(3~{R})-8-methoxy-3-methyl-3-oxidanyl-2,4-dihydrobenzo[a]anthracene-1,7,12-trione 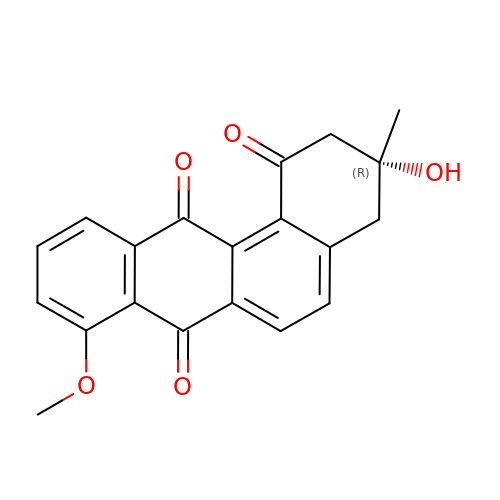| C20 H16 O5 | XZLGWJORNHETKI-HXUWFJFHSA-N> AVSLDRTRAVFDGSEKSMTLDISNDNKQLPYLAQAWIENENQEKIITGPVIATPPVQRLEPGAKSMVRLSTTPDISKLPQDRESLFYFNLREIPPRSEKANVLQI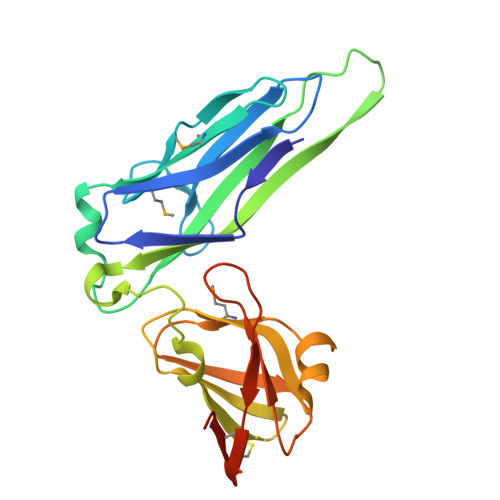ALQTKIKLFYRPAAIKTRPNEVWQDQLILNKVSGGYRIENPTPYYVTVIGLGGSEKQAEEGEFETVMLSPRSEQTVKSANYNTPYLSYINDYGGRPVLSFICNGSRCSVKKEKHHHHHH>SLEHHHHHHENLYFQSGTRWAVLVAGSSGYWNYRHQADICHAYQLLRKGGLKEENIVVFMYDDIANNYENPRPGTIINSPHGKDVYQGVPKDYTGDDVNVDNLFAVILGDKTAVKGGSGKVVDSGPNDHIFIFYSNHGGPGVLGMPTSPYLYANDLNDVLKKKHALGTYKSLVFYLEACESGSIFEGLLPEGLNIYATTASNAEESSWGTYCPGEEPSPPPEYETCLGDLYSVAWMEDSGMHNLQTETLHQQYELVKRRTAPVGYSYGSHVMQYGDVGISKDNLDLYMGTNPANDNFTFADANSLKPPSRVTNQRDADLVHFWEKYRKAPEGSARKTEAQKQVLEAMSHRLHIDNSVILVGKILFGISRGPEVLNKVRSAGQPLVDDWNCLKNQVRAFERHCGSLSQYGIKHMRSFAN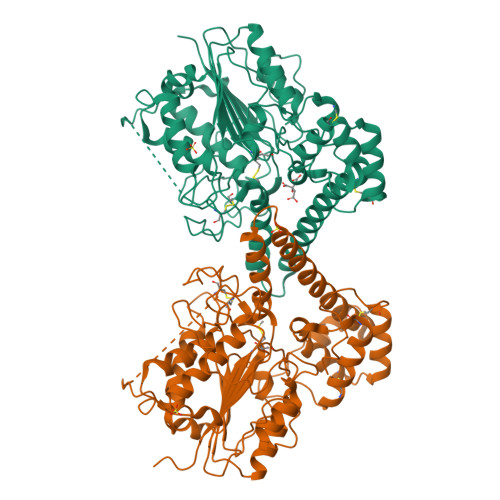ICNAGIQMEQMEEAASQACTTLPTGPWSSLNRGFSA[4x]>MEEIQGYDVEFDPPLESKYECPICLMALREAVQTPCGHRFCKACIIKSIRDAGHKCPVDNEILLENQLFPDNFAKREILSLMVKCPNEGCLHKMELRHLEDHQAHCEFALMDCPQCQRPFQKFHINIHILKDCPRRQVSCDNCAASMAFEDKEI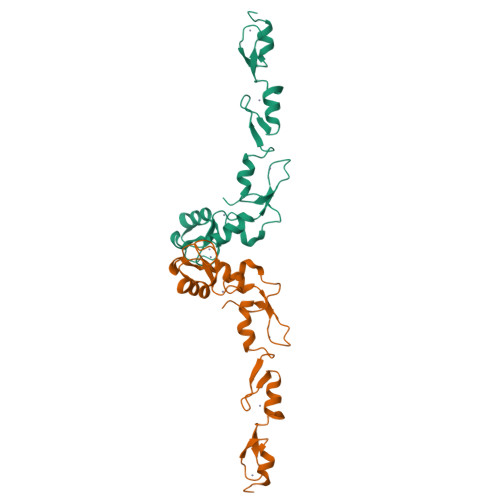HDQNCPLALEHHHHHH[2x]>GSHMIKPDETRVKQFLEGFNIETFEMVGTLSNAQGTFALVKGAGGVHRVRVGDYLGRNDGKVVGISE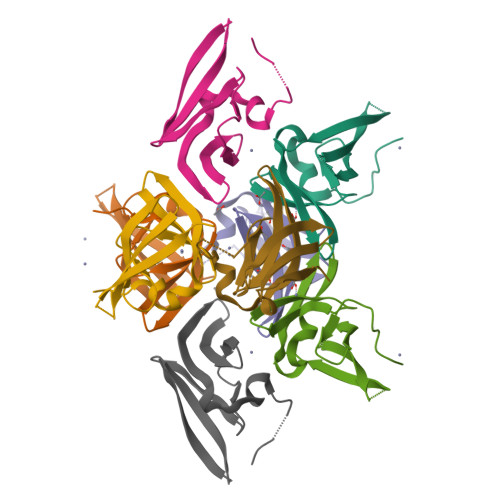GKIDVIEIVPDGEGNWLERPRSLTLK[4x]> MNILQEPIDFLKKEELKNIDLSQMSKKERYKIWKRIPKCELHCHLDLCFSADFFVSCIRKYNLQPNLSDEEVLDYYLFAKGGKSLGEFVEKAIKVADIFHDYEVIEDLAKHAVFNKYKEGVVLMEFRYSPTFVAFKYNLDIELIHQAIVKGIKEVVELLDHKIHVALMCIGDTGHEAANIKASADFCLKHKADFVGFDHGGHEVDLKEYKEIFDYVRESGVPLSVHAGEDVTLPNLNTLYSAIQVLKVERIGHGIRVAESQELIDMVKEKNILLEVCPISNVLLKNAKSMDTHPIR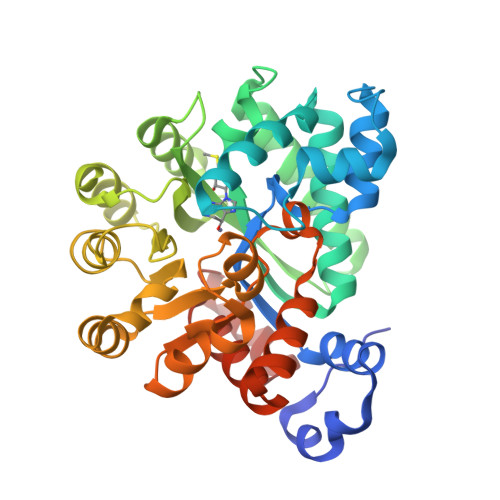QLYDAGVKVSVNSDDPGMFLTNINDDYEELYTHLNFTLEDFMKMNEWALEKSFMDSNIKDKIKNLYFKGEFEAYV>MIGPRLCAATPRFPLVSLAHRNSKVFALASSNAVAQRWGKRFYAPIETETPHKVGVEFEESKDRIFTSPQKYVQGRHAFTRSYMYVKKWATKSAVVLADQNVWNICANKIVDSLSQNGMTVTKLVFGGEASLVELDKLRKQCPDDTQVIIGVGGGKTMDSAKYIAHSMNLPSIICPTTASSDAATSSLSVIYTPDGQFQKYSFYPLNPNLIFIDTDVIVRAPVRFLISGIGDALSTWVETESVIRSNSTSFAGGVASIAGRYIARACKDTLEKYALSAILSNTRGVCTEAFENVVEANTLMSGLGFENGGLAAAHAIHNGMTAIHGPVHRLMH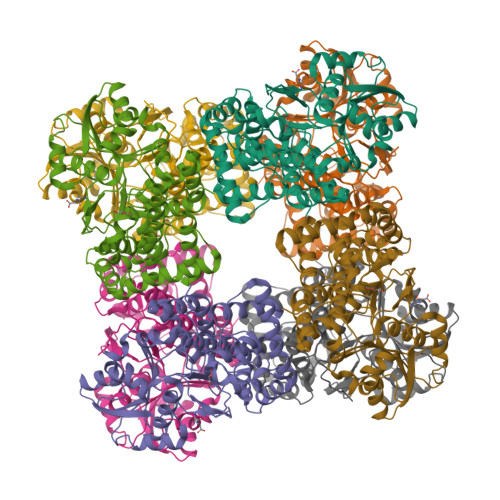GEKVAYGTLVQVVLEDWPLEDFNNLASFMAKCHLPITLEELGIPNVTDEELLMVGRATLRPDESIHNMSKKFNPSQIADAIKAVDSYSQKWQEQTGWTERFRLPPSRHSPHLTDIHP[2x]~{N}-[(3~{S})-7,9-bis(fluoranyl)-2-oxidanylidene-1,3,4,5-tetrahydro-1-benzazepin-3-yl]-3-(phenylmethyl)-1~{H}-1,2,4-triazole-5-carboxamide 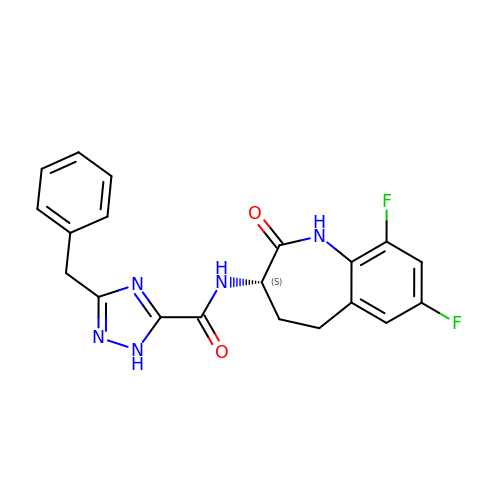| C20 H17 F2 N5 O2 | ATQAGKAMBISZQM-HNNXBMFYSA-N>[2x]NSAITKANGENNAVVKINKTLNIAEGITTPTATFTFKFTEKTGQSSNGAPYQTGVAIPDRNVEYNKNDHPTADKIQKATEDIFSGVAYGHAGEYVYDVAEAKTGWQAITKNGKTIDAMRYDKRTYEMHVIVKNKVNGGVYISSVYFKENNKSNAPKVESSEQGVYNLFDNTYTKDASKEPNPDDPSQVDPNAKALTITKKVDGASGDKTRDFQFHIKIQLPSTNKTAETPVTNI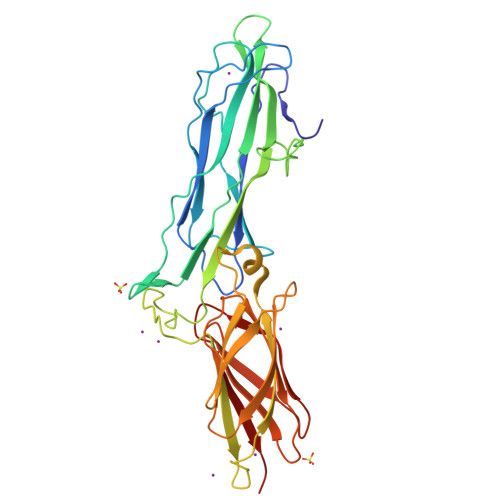IVKHGSKSEVLAVVTPADTVEYNFTLKDGETFTVEQLPAGSKYTVTETGVAGYTDSSIYTTNGAEQTSQGQKNVDFTLTDILIGEKKNDNKVTNKIDD> MLKAWHLPVAPFIKEQQERLMITLWLSGDDLPPRVTLRAEEDNEELSLPMHRLRQAPHPGVVAWRGEINLVNGQPRRRYSFKLLWADRQLWFTPQEFNRFPPARLEQFAVDLPDSGPQWVADQVFYQIFPDRFARSQSREAEQDATYYHHAAGHDIVRKAWDEPLTAEAGGSTFYGGDLDGISEKLPYLKQLGVTALYLNPVFVAPSVHKYDTEDYRRVDPQFGGDAALLRLRHNTQKEGMRLILDGVFNHSGDSHAWFDRHQRGSGGACHNADSPWRDWYNFSPEGVAHDWLGYASLPKLDYRSSTLIDEIYGGEDSVVRHWLKAPWSMDGWRLDVVHMLGEGGGARNNLRHIAGITQAAKLERPDAFVFGEHFGDARQWLQADVEDSAMNYRGFTFPLWGFLANTDISYDPQKIDAQTCMAWMDNYRAGLSHQQQLRMFNQLDSHATARFKSLLGKDVARLPLAVVWLFSWPGVPCIYYGDEVGVDGNNDPFCRKPFPWDPALQDGDLLDLYKRMSKLRKAHQALRYGGCQVIYAEDNVVVFVRVYKQQRVLVAINRGEACEVVIEDSPLL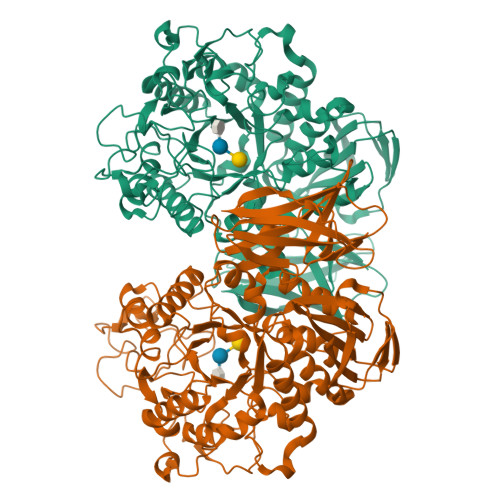DVNGWQLKEGAGALHDGVLTLPAISASVWFSR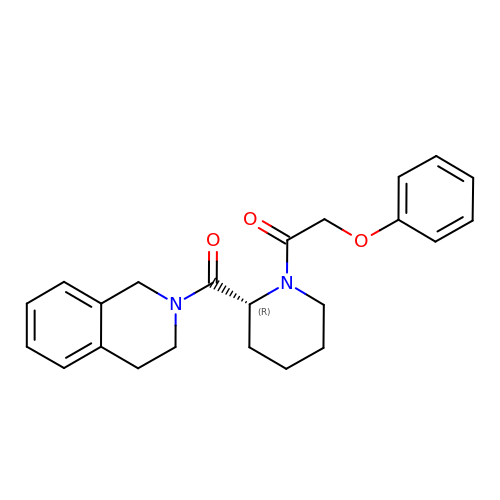1-[(2R)-2-(3,4-dihydroisoquinolin-2(1H)-ylcarbonyl)piperidin-1-yl]-2-phenoxyethanone | C23 H26 N2 O3 | CJQMUNJPWNNVDR-OAQYLSRUSA-N>PLREAKDLHTALHIGPRALSKASNISMQQAREVVQTCPHCNSAPALEAGVNPRGLGPLQI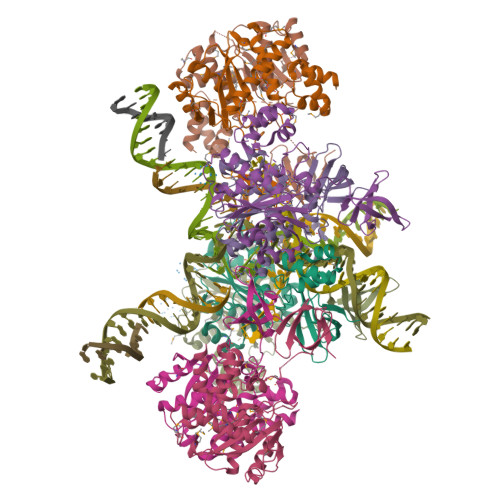WQTDFTLEPRMAPRSWLAVTVDTASSAIVVTQHGRVTSVAVQHHWATAIAVMGRPKAIKTDNGSCFTSKSTREWMARWGIAHTTGIPGNSQGQAMVERANRMMKDKIRVLAEGDGFMKRIPTSKQGEMMAKAMYALNHFERGENTKTPIQKHWRPTVLTEGPPVKIRIETGEWEKGWNVLVWGRGYAAVKNRDTDKVIWVPSRKVKPDIT[8x]> DPF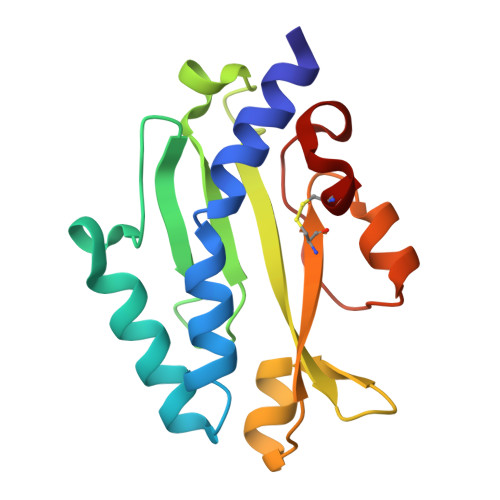TVRTRVSEGLVLAEPAKLMISTDGSASTADLTRATTTWNQQSNNLGASSKYVTSVLMDAGNTGVITITYVADQVGLPTAGNTLILSPYINDGNTRTALATAVAAGTRGTIDWACTSASNATATAQGFTGMAAGSVPQEFAPAQCR>[2x]MSVKTKEKEMAVTILYEQDVDPKVIQGLKVGIIGYGSQGHAHALNLMDSGVDVRVGLREGDSDWKTAEEAGLKVTDMDTAAEEADVIMVLVPDEVQPKVYQEHIAAHLKAGNTLAFAHGFNIHYGYIVPPEDVNVIMCA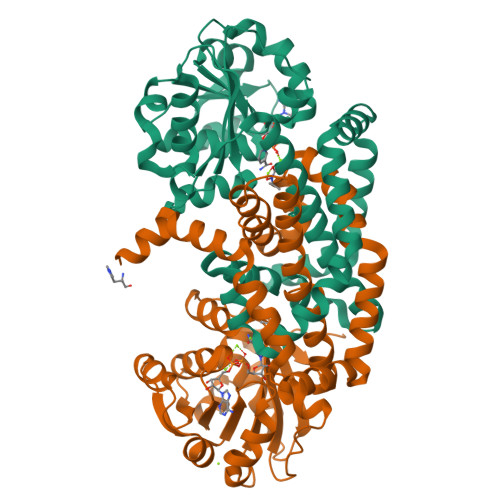PKGPGHIVRRQFTEGSGVPDLACVQQDATGNAWDIVLSYCWGVGGARSGIIKATFAEETEEDLFGEQAVLCGGLVELVKAGFETLTEAGYPPELAYFECYHEMKMIVDLMYESGIHFMNYSISNTAEYGEYYAGPKVINEQSREAMKEILKRIQDGSFAQEFVDDCNNGHKRLLEQREAINTHPIETTGAQIRSMFSWIKKEDLEHHHHHH> MSSEFISKVDKEARRKAANILRDKFLNLVEQLKKGEPLVMEIPMRTLSNAIYDEKRKLLLLGEKKLRRNFLDLNEAKRFMQTVLMASIIYDALVSDEYPTIRDLYYRGKHSLLLKSIEGNKIVSEENTWDEQKESDSVIVDIEVFTSLLREEMLILSKEKGKVVGNLRIRSGNDVIDLSKTGHGAYAIEPTPDLIDFIDVDAEFVLVVEKDAVFQQLHRAGFWKQYKSILITSAGQPDRATRRFV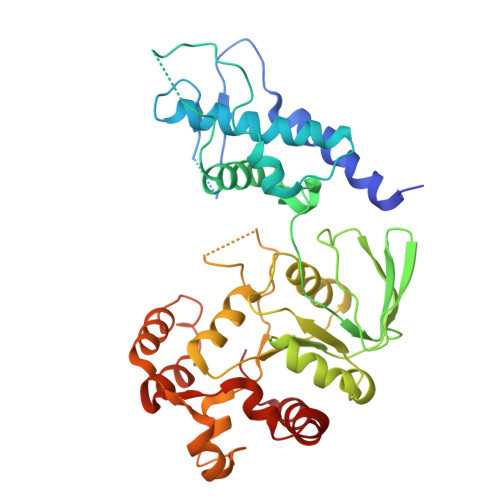RRLNEELKLPVYILTDADPYGWYIFSVFRIGSISLSYESERLATPDAKFLGVSMGDIFGNSRKKPYLSEAERKNYIIKAKDADIKRAEEIKNYEWFKTKAWQEEINTFLQRKAKLEIEAMASKGLKFLAFQYIPEKITNKDYIA>KVFSKCELAHKLKAQEMDGFGGYSLANWVCMAEYESNFNTRAFNGKNANGSYDYGLFQLNSKWWCKDN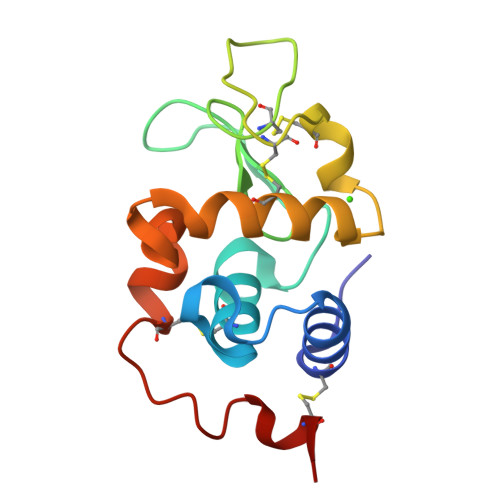KRSSSNACNIMCSKLLDDNIDDDISCAKRVVRDPKGMSAWKAWVKHCKDKDLSEYLASCNL[2x]> MNEDLPKEYFELIRKALNEKEAEKAPLSRRRRVRRKNQPLPDAKKKFKTGLNELPRESVVTVNLDSSDDGVVTVPTDDSVEEIQSSEEDYDSEEFEDVTDGNEVAGVEDISVEIKPSSKRNSDARRTSRNVCSNEERKRRKYFHMLYLVCLMVHGFIRNEWINSKRLSRKLSNLVPEKVFELLHPQKDEELPLRSTRKLLDGLKKCMELWQKHWKITKKYDNVGLYMRTWKEIEMSANNKRKFKTLKRSDFLRAVSKGHGDPDISVQGFVAMLRACNVNARLIMSCQPPDFTNMKIDTSLNGNNAYKDMVKYPIFWCEVWDKFSKKWITVDPVNLKTIEQVRLHSKLAPKGVACCERNMLRYVIAYDRKYGCRDVTRRYAQWMNSKVRKRRITKDDFGEKWFRKVITALHHRKRTKIDDYEDQYFFQRDESEGIPDSVQDLKNHPYYVLEQDIKQTQIVKPGCKECGYLKVHGKVGKVLKVYAKRDIADLKSARQWYMNGRILKTGSRCKKVIKRTVGRPKGEAEEEDERLYSFEDTELYIPPLASASGEITKNTFGNIEVFAPTMIPGNCCLVENPVAIKAARFLGVEFAPAVTSFKFERGSTVKPVLSGIVVAKWLREAIETAIDGIEFIQEDDNRKEHLLGALESWNTLLLKLRIRSKLNSTYGKIAEEEPNVTKEQNIADNHDNTETFMGGGFLPGIANHEARPYSEPSEPE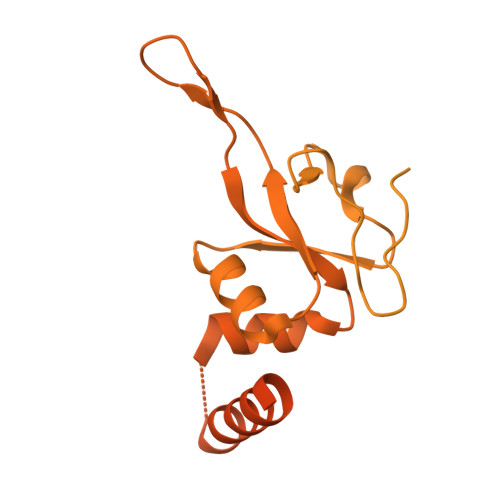DSLDYVSVDKAEESATDDDVGEDYSDFMKELEMSEESD> MGHHHHHHGSTELTPDQQTLLHFIMDSYNKQRMPQEITNKILKEAFSAEENFLILTEMATNHVQVLVEFTKKLPGFQTLDHEDQIALL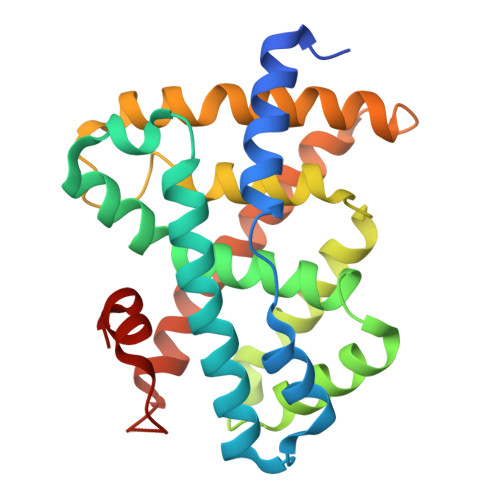KGSAVEAMFLRSAEIFNKKLPSGHSDLLEARIRNSGISDEYITPMFSFYKSIGELKMTQEEYALLTAIVILSPDRQYIKDREAVEKLQEPLLDVLQKLCKIHQPENPQHFACLLGRLTELRTFNHHHAEMLMSWRVNDHKFTPLLCEIWDVQ> MAHHHHHHSSGLEVLFQGPNEQVSRSQQRGLRRVRDLCRVLQLPPTFEDTAVAYYQQAYRHSGIRAARLQKKEVLVGCCVLITCRQHNWPLTMGAICTLLYADLDVFSSTYMQIVKLLGLDVPSLCLAELVKTYCSSFKLFQASPSVPAKYVEDKEKMLSRTMQLVELANETWLVTGRHPLPVITAATFLAWQSLQPADRLSCSLARFCKLANVDLPYPASSRLQELLAVLLRMAEQLAWLRVLRLDKRSVVKHIGDLLQHRQSLVRSAFRDGTAEVETREKEPPGWGQ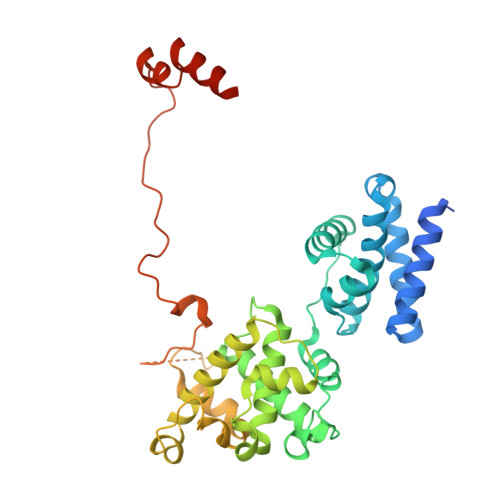GQGEGEVGNNSLGLPQGKRPASPALLLPPCMLKSPKRICPVPPVSTVTGDENISDSEIEQYLRTPQEVRDFQRAQAARQAATSVPNPP>[4x]MLRHLAGASALALTLAGAGFAQDHDHDHEDVTLYRVFVGDHE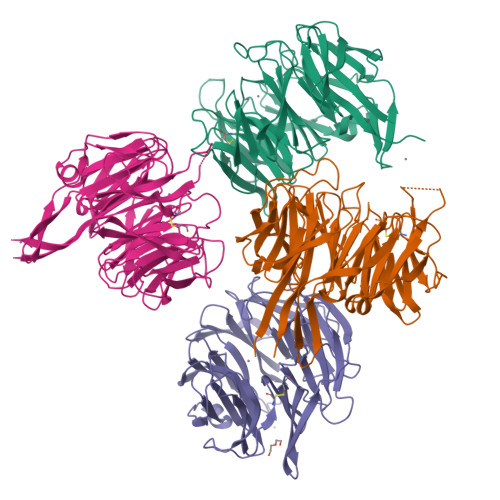KGQVTAFDLAEPDHRWTFPTTGQVKLYSVAGGAVVAAVQSDADTVQFIRSGISFHDHGDHRDIEVGDPAAIDASLTGPRPFHLVEHDGKVVLNYDQGGYAEILDGHALAEGKAEPGRFPQARAHHGFVAPLGGNWLSTVASDEKVEGDASVPRLGLQAFDAEGNPAGNLATCTGIHGEAFSGAYLAAGCKEGVLTVKAGANGSEYKLLPYPADLPQGVTTGTLLGSTGIQVFLGNYGPDGLVVIDPVDEPHYRYIKLPFRRVDFALDPAKPSTGYVLTEDGSLHRIDLLKAEIVASAKVTEPYSMDGHWNDPRPRIAMAGDEIVVTDPNAGLVRRIATEDLSERGTVPVEGKPYNIAVTGGSGVTH The activity of H3K4-specific modification enzymes, in higher eukaryotes the MLL (or KMT2) family, is tightly regulated. All contain a catalytic SET domain that associates with a core multiprotein complex for activation. A defining feature of the MLL family, conserved through evolution, is that their SET domain must associate with a multiprotein complex for full catalytic activity (Dehe et al., 2006; Dou et al., 2006; Roguev et al., 2001; Yokoyama et al., 2004). Here we show that, unlike MLL1, the MLL4 SET domain retains significant activity without the core complex.

The final construct used for structural determination, MLL4(tag), encompassed residues 5,384 to 5,536, followed by a C-terminal 6xHis tag, and crystallized with S-adenosylhomocysteine (SAH) cofactor product. The crystals diffracted to a resolution of 2.2 Å and belonged to the space group P21. The catalytic domain of MLL4(tag) adopts the canonical β-fold structure observed for other SET domains, and closely resembles that of MLL1 (Dillon et al., 2005; Southall et al., 2009; Xiao et al., 2003b). The N-flanking region of MLL4 forms an extended helical structure, and is markedly different from the extended loop observed for MLL1. The C-terminal tag immediately follows the conserved Cys4Zn cluster and enters the substrate binding channel before turning and passing over the cofactor. The lack of methyltransferase activity observed with the C-terminally tagged construct can be attributed to partial blocking of the substrate binding channel and interactions with the cofactor. In MLL4(tag) the SET-I region, which retains the conserved fold observed in MLL1 and other SET domain structures, is in a position that is more consistent with the “closed” conformation proposed for an active SET domain (Southall et al., 2009). The consequence of this position for the MLL4 SET-I region is that the four-residue motif, termed the channel tetrapeptide (I-Y-M-F in MLL4), is 3.3 Å closer to the conserved active-site tyrosine that flanks the target lysine side chain (Tyr5512 residue in MLL4) relative to MLL1. Inspection of the MLL4 structure reveals that several side chains of residues in the postSET loop are oriented toward the SET-I region, and some are capable of making hydrogen bonds with it. From this we infer that when associated with WRAD, both proteins adopt a similar optimal conformation when fully activated. This implies that the structure of the isolated MLL4 SET domain, with respect to the positions of the SET-I region and postSET loop, may represent an intermediate state, which is partially stabilized by features unique to MLL4.

> MTLHSKSSQYRRLRTEWKNNVYLARSRIQGLGLYAAKDLEKHTMVIEYIGTIIRNEVANRREKIYEEQNRGIYMFRINNEHVIDATLTGGPARYINHSCAPNCVAEVVTFDKEDKIIIISSRRIPKGEELTYDYQFDFEDDQHEIPCHCGAWNCRKWMKGHHHHHH(1~{S},2~{R},3~{R},4~{S},5~{S})-4-[[4-[3-(1-adamantylmethoxy)propyl]-1,2,3-triazol-1-yl]methyl]cyclohexane-1,2,3,5-tetrol 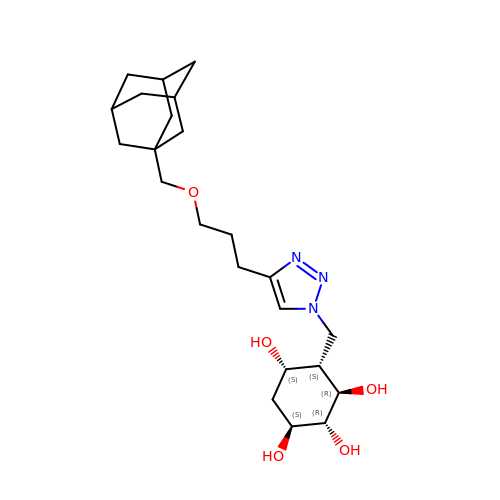| C23 H37 N3 O5 | SADPKFATELTVOP-HXOWLEFZSA-N>[2x]PQFSLWKRPVVTAYIEGQPVEVL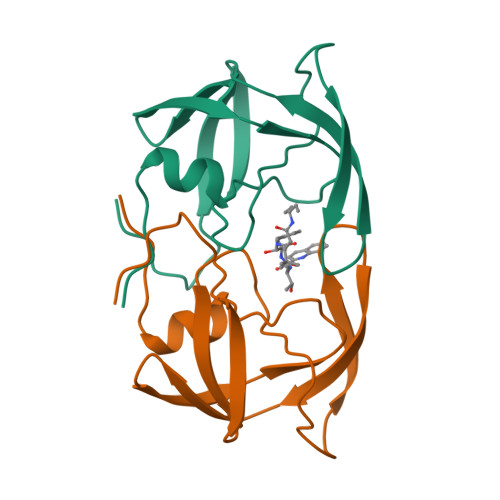LDTGADDSIVAGIELGNNYSPKIVGGIGGFINTKEYKNVEIEVLNKKVRATIMTGDTPINIFGRNILTALGMSLNL>[2x]MATQEEILDAALVSGDSSQLTDSHLVALRLQQQVERIRQTRTQLLDGLYQNLSQAYDPGAASMWVLPANPDNTLPFLIGDKGRVLASLSLEAGGRGLAYGTNVLTQLSGTNAAHAPLLKRAVQWLVNGDPGAATAKDFKVSVVGVDKTAALNGLKSAGLQPADAACNALTDASCASTSKLLVLGNGASAASLSATVRARLQAGLPILFVHTNGWNQSSTGQQILAGLGLQEGPYGGNYWDKDRVPSSRTRTRSVELGGAYGQDPALVQQIVDGSWRTDYDWSKCTSYVGRTTCDDVPGLSDFSKRVDVLKGALDAYNQKAQNLFALPGTTSLRLWLLWADAVRQNIRYPMDKAADTARFQETFVADAIVGYVREAGAAQKELGSYAGQRQQSMPVSGSEETLTLTLPSAQGFTAIGRMAAPGKRLSIRIEDAGQASLAVGLNTQRIGSTRLWNTRQYDRPRFLKSPDIKLQANQSVALVSPYGGLLQLVYSGATPG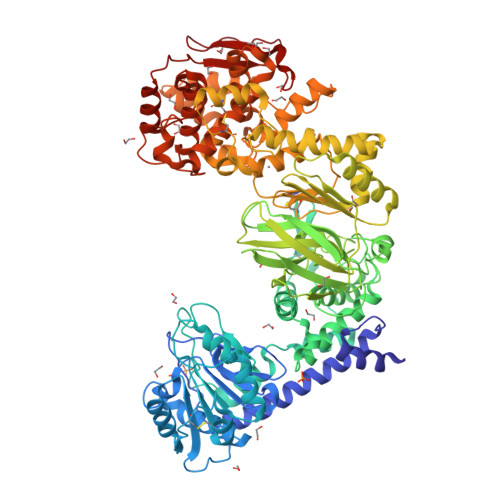QTVTVKVTGAASQPFLDIQPGEDSSQAIADFIQALDADKADWLEIRSGSVEVHAKVEKVRGSIDKDYGGDVQRFIRELNEVFIDDAYTLAGFAIPNQAKTPAIQQECAARGWDCDSETLHKLPGTQHINVDQYAQCGGGCSGNPYDQTWGLNPRGWGESHELGHNLQVNRLKVYGGRSGEISNQIFPLHKDWRVLREFGQNLDDTRVNYRNAYNLIVAGRAEADPLAGVYKRLWEDPGTYALNGERMAFYTQWVHYWADLKNDPLQGWDIWTLLYLHQRQVDKSDWDANKAALGYGTYAQRPGNSGDASSTDGNDNLLLGLSWLTQRDQRPTFALWGIRTSAAAQAQVAAYGFAEQPAFFYANNRTNEYSTVKLLDMSQGSPAWPFPLE> MQDAITAVINSADVQGKYLDGAAMDKLKSYFASGELRVRAASVISANAATIVKEAVAKSLLYSDVTRPGGNMYTTRRYAACIRDL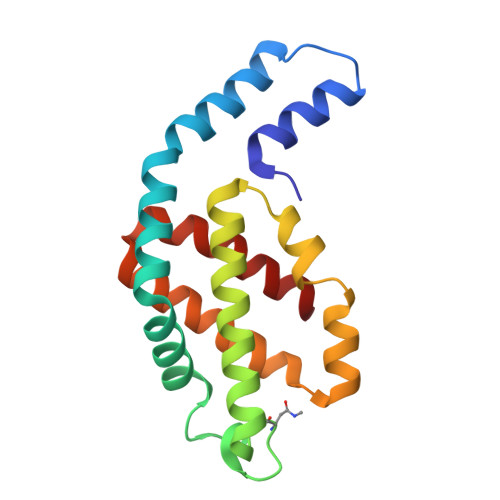DYYLRYATYAMLAGDASILDERVLNGLKETYNSLGVPISSTVQAIQAIKEVTASLVGADAGKEMGVYLDYICSGLS> GAQVSRQNVGTHST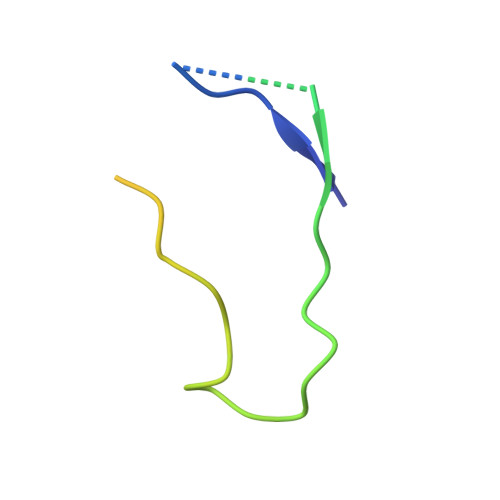QNSVSNGSSLNYFNINYFKDAASNGASKLEFTQDPSKFTDPVKDVLEKGIPTLQ>[2x]GPLG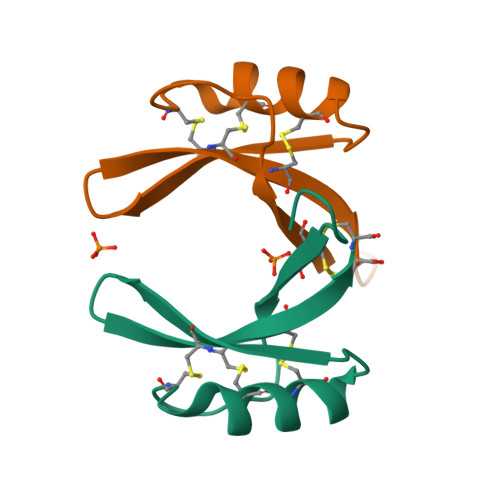SRHCLSQSHRFKGMCVSSNNCANVCRTESFPDGECKSHGLERKCFCKKVC>MQLRFARLSEHATAPTRGSARAAGYDLYSAYDYTIPPMEKAVVKTDIQIALPSGCYGRVAPRSGLAAKHFIDVGAGVIDEDYRGNVGVVLFNFGKEKFEVKKGDRIAQLICERIFYPEIEEVQALDDT[3x];>MAELPTHYGTIIKTLRKYMKLTQSKLSERTGFSQNTISNHENGNRNIGVNEIEIYGKGLGIPSYILHRISDEFKEKGYSPTLNDFGKFDKMYSYVNKAYYNDGDIYYSSYDLYDETIKLLELLKESKINVNDIDYDYVLKLYKQILS[3x]

The dUTPase enzyme plays a key role in preventive DNA repair by eliminating dUTP from the DNA biosynthetic pathway, meanwhile it also produces dUMP, a precursor for dTTP biosynthesis. The lack of dUTPase activity leads to high cellular dUTP level, and increases the frequency of uracil incorporation into the genome upon synthesis or repair as most polymerases do not discriminate dUTP over dTTP4,5. Overwhelming of the uracil base excision repair mechanism by perturbing the function of dUTPase induces DNA fragmentation and cell death. In 2010 it was discovered that φ11 and 80α bacteriophage dUTPases interact with the staphylococcal Stl protein involved in the regulation of a Staphylococcus aureus pathogenicity island.

On one hand, we determined the complex of hDUT with the crystallizable amino terminal domain of Stl (StlNT) by X-ray crystallography. The complex was crystallized in P212121 space group, and the asymmetric unit contains a trimer dUTPase bound to three StlNT chains. Based on our hydrogen deuterium exchange mass spectrometry (HDX-MS) results a short segment of Stl binds to the active site of φ11 phage and human dUTPase blocking the pocket from the substrate. Based on HDX-MS and 3D crystal structures a peptide segment of Stl including residues 106–113 directly binds to the active site of the enzyme. In case of the phage DUT-StlNT complex the N-terminal of the dUTPase (residues: R15, E18, N20, H21, D24) serves as a secondary interaction surface with Stl (residues D77, R74, Y70 and Y98, N102, Y106 respectively). These interactions are missing in case of hDUT and LvDUT, as the residues in the matching positions are unable to interact with Stl. In case of φ11 phage dUTPase sidechain of Stl-Y106 forms H-bond interactions with the N-terminal of the enzyme (residues H21, D24), while it has no detectable interaction with hDUT. Based on the crystal structure of StlNT, residues to be mutated (i.e. V55, Y106, S114, Y116) are found on the surface of the protein forming no sidechain interactions with the core of the protein, with the exception of the sidechain of S114, which interacts with the mainchain of D110. We showed that the C-terminal part of the Stl protein omitted from the crystal structure has an important role in the enzyme inhibition as the full-length Stl is needed to exert maximal inhibition on the human dUTPase.> EPAENSDFYLPGDYLLGGLFSLHANMKGIVHLNFLQVPMCKEYEVKVIGYNLMQAMRFAVEEINNDSSLLPGVLLGYEIVDVCYISNNVQPVLYFLAHEDNLLPIQEDYSNYSSRVVAVIGPDNSESVMTVANFLSLFLLPQITYSAISDELRDKVRFPALLRTTPSADHHIEAMVQLMLHFRWNWIIVLVSNDTYGRDNGQLLGERVARRDICIAFQETLPTLQPNQNMTSEERQRLVTIVDKLQQSTARVVVVFSPDLTLYHFFNEVLRQNFTGAVWIASESWAIDPVLHNLTELRHLGTFLGITIQSVPIPGFSEFREWGPQAGPPPLSRTSQSYTCNQECDNCLNATLSFNTILRLSGERVVYSVYSAVYAVAHALHSLLGCDKSTCTKRVVYPWQLLEEIWKVNFTLLDHQIFFDPQGDVALHLEIVQWQWDRSQNPFQSVASYYPLQRQLKNIQDISWHTINNTIPMSMCSKRCQSGQKKKPVGIHVCCFECIDCLPGTFLNHTEDEYECQACPNNEWSYQSETSCFKRQLVFLEWHEAPTIAVALLAALGFLSTLAILVIFWRHFQTPIVRSAGGPMCFLMLTLLLVAYMVVPVYVGPPKVSTCLCRQALFPLCFTICISCIAVRSFQIVCAFKMASRFPRAYSYWVRYQGPYVSMAFITVLKMVIVVIGMLATGLSPTTRTDPDDPKITIVSCNPNYRNSLLFNTSLDLLLSVVGFSFAYMGKELPTNYNEAKFITLSMTFYFTSSVSLCTFMSAYSGVLVTIVDLLVTVLNLLAISLGYFGPKCYMILFYPERNTPAYFNSMIQGYTMRRD;> LCLSQQFKAQGDYILGGLFPLGSTEEATLNQRTQPNSIPCNRFSPLGLFLAMAMKMAVEEINNGSALLPGLRLGYDLFDTCSEPVVTMKSSLMFLAKVGSQSIAAYCNYTQYQPRVLAVIGPHSSELALITGKFFSFFLMPQVSYSASMDRLSDRETFPSFFRTVPSDRVQLQAVVTLLQNFSWNWVAALGSDDDYGREGLSIFSSLANARGICIAHEGLVPQHDTSGQQLGKVLDVLRQVNQSKVQVVVLFASARAVYSLFSYSIHHGLSPKVWVASESWLTSDLVMTLPNIARVGTVLGFLQRGALLPEFSHYVETHLALAADPAFCASLNAELDLEEHVMGQRCPRCDDIMLQNLSSGLLQNLSAGQLHHQIFATYAAVYSVAQALHNTLQCNVSHCHVSEHVLPWQLLENMYNMSFHARDLTLQFDAEGNVDMEYDLKMWVWQSPTPVLHTVGTFNGTLQLQQSKMYWPGNQVPVSQCSRQCKDGQVRRVKGFHSCCYDCVDCKAGSYRKHPDDFTCTPCNQDQWSPEKSTACLPRRPKFLAWGEPVVLSLLLLLCLVLGLALAALGLSVHHWDSPLVQ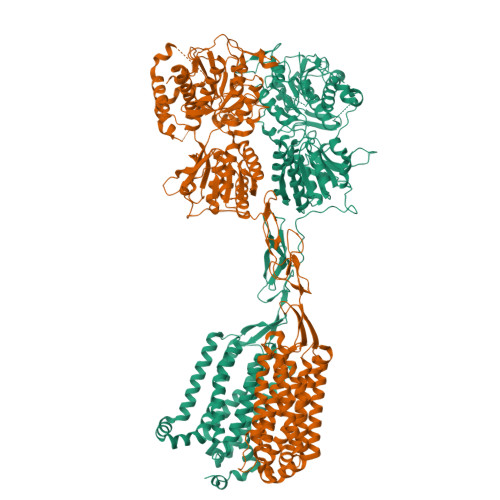ASGGSQFCFGLICLGLFCLSVLLFPGRPSSASCLAQQPMAHLPLTGCLSTLFLQAAETFVESELPLSWANWLCSYLRGLWAWLVVLLATFVEAALCAWYLIAFPPEVVTDWSVLPTEVLEHCHVRSWVSLGLVHITNAMLAFLCFLGTFLVQSQPGRYNRARGLTFAMLAYFITWVSFVPLLANVQVAYQPAVQMGAILVCALGILVTFHLPKCYVLLWLPKLNTQEFFL>[5x]MKTINSVDTKEFLNHQVANLNVFTVKIHQIHWYMRGHNFFTLHEKMDDLYSEFGEQMDEVAERLLAIGGSPFSTLKEFLENASVEEAPYTKPKTMDQLMEDLVGTLELLRDEYKQGIELTDKEGDD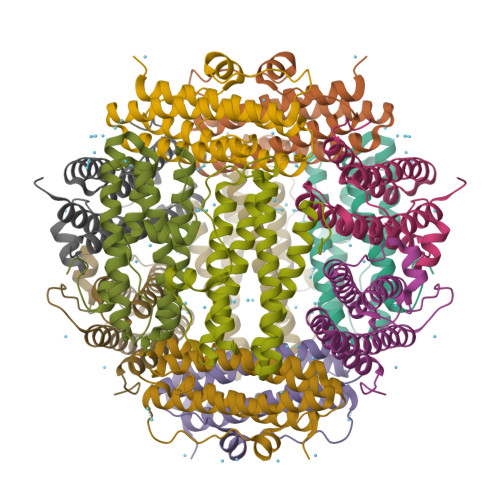VTNDMLIAFKASIDKHIWMFKAFLGKAPLE;> MKTINSVDTKEFLNHQVANLNVFTVKIHQIHWYMRGHNFFTLHEKHDDLYSEFGEQMDEVAERLLAIGGSPFSTLKEFLENASVEEAPYTKPKTMDQLMEDLVGTLELLRDEYKQGIELTDKEGDDVTNDMLIAFKASIDKHIWMFKAFLGKAPLE> GPGSLGSGAYR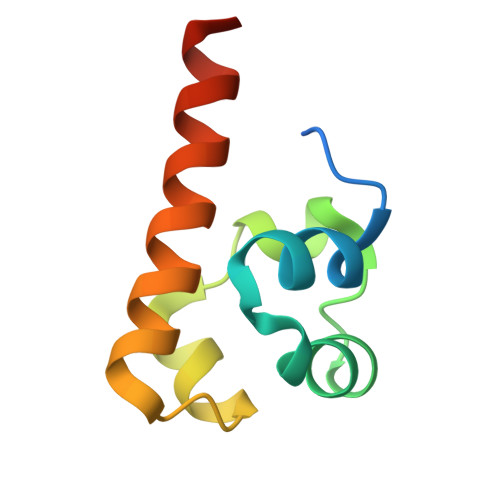SVGEWLEAIKMGRYTEIFMENGYSSMDAVAQVTLEDLRRLGVTLVGHQKKIMSSLQEMKVQMVNGMVPV The Hanks-type Ser/Thr protein kinase (STPK) PknG and its FHA (ForkHead-Associated) substrate OdhI (Oxoglutarate dehydrogenase Inhibitor) are at the core of a conserved signal transduction pathway that modulates central metabolism in distant actinobacteria. Both in Corynebacterium glutamicum, a soil bacterium used for the industrial production of amino acids, and in the pathogen Mycobacterium tuberculosis, PknG modulates the 2-oxoglutarate dehydrogenase activity in the Krebs cycle by controlling the phosphorylation status of the regulator OdhI (called GarA in the genus Mycobacterium). PknG has a unique modular organization characterized by the presence of a highly flexible N-terminal region containing all known autophosphorylation sites and a C-terminal domain composed of tetratricopeptide repeats (TPRs) flanking the kinase catalytic core. To investigate the conservation of mechanisms involved in the regulation of PknG, we studied the kinase isoform from C. glutamicum (CgPknG), which is devoid of an Rdx domain.

To investigate the structural basis of the regulation of a PknG isoform lacking an Rdx domain, we solved a high-resolution crystal structure of CgPknG in complex with the nonhydrolyzable ATP analog AMP-PNP. The final atomic model contains two copies of CgPknG within the asymmetric unit, encompassing residues 123 to 799 and 125 to 798, respectively, including a short fragment of the N-terminal region, the kinase catalytic core and the TPR domain. In addition, mFo–DFc sigma-A-weighted electron density maps clearly revealed the bound nucleotide and two Mg(II) atoms at the active site of each CgPknG molecule. Notably, even though we used full-length CgPknG in our crystallization assays, we found no evidence for residues 1 to 122 in electron density maps. Edman degradation experiments revealed that the N-terminal residue of crystallized CgPknG was Val123, suggesting that the kinase N-terminal segment was partially degraded during crystal growth and that, as similarly reported for MtbPknG, it is probably unstructured in most of its length. The absence of extensive protein-protein interactions in the crystal structure suggests that the protein is monomeric in solution, in agreement with analytical ultracentrifugation data. CgPknG and MtbPknG share the same overall fold and topology, except for the absence of a regulatory Rdx domain in CgPknG that leads to a more accessible active site. Also similar to MtbPknG, most functionally important and conserved motifs in the active site of CgPknG exhibit conformations compatible with a standard eukaryotic protein kinase active state, and the activation loop is stabilized in an open and extended conformation, permissive for substrate binding in the absence of phosphorylation. Nevertheless, CgPknG residue Glu222 is found away from the catalytic Lys205, pointing out of the active site due to an outward conformation of the helix αC, as previously reported for MtbPknG.

>VRRQSRPVADGMVELPFITPKPEDELLIDPEKKRKPGVAAPQLVAGDIVAEQYEVLGVIAHGGMGWIYLANDRNVSGRIVVLKGMMAQSSVQDQGTAEAEREFLADITHPGIVKAYNFIDDPRVPGGFIVMEYVNGPSLKDRCKAQPDGVLRVDLAIGYILELLPAMDYLHQRGVVYNDLKPENVIATEDQVKLIDLGAVTGIGAFGYIYGTKGFQAPEVATHGPSISSDIFTIGRTLAALTMPLPVEDGVLAPGIPSPKNSPLLRRHLSFYRLLQRATADDPQHRFRNVSELRTQLYGVLREILAVRDGKQYPPQHSLFSPQRSTFGTKHLVFRTDRIIDGIERQARITAPEIVSALPVPLIDRTDPGARMLSGSSYAEPSETLETLRNSMEDEQYRQSIEIPLGVVRALLDLGFTTEARQWLETLEGRIGDDWRHKWFSGITYLLLDDYATAQVFFNHVLTILPGEAAPKLALAAVDELILQQIGAESTAYLTPDIVSATATLSKDFEDLDASAFESLSDTWSHISSDPHVVRFHSLRLYALVWATNPTTVSSAFGLARQLMAENQIELAVQALDKLPQSSTHYRMATLTTILLLVSSNLSESRIRRAARRLTEIPTNEPRFNQIKIAIMSAGLSWLRERKLKASASANPLFEYPFSQKGLRTGISEALRIQARSAPFPHHRYALVDMANAVRPLSWF[2x]> ADVGSCSVGNNPLAQLHKHTQQNKSLQFNQKNNGRLNESPLQGTNKPGISEAFISNVNAISQENMANMQRFINGEPLIDDKRRMEIGPSSGRLPPFSNVHSLQTSANPTQIKGVNDISHWSQEFQGSNSIQNRNADTGNSEKAWQRGSTTASSRFQYPNTMMNNYAYASMNSLSGSRLQSPAFMNQQQSGRSKEGVNEQEQQPWTDQFEKLEKEVSENLDINDEIEKEENVSEVEQNKPETVEKEEGVYGDQYQSDFQEVWDSIHKDAEEVLPSELVNDDLNLGEDYLKYLGGRVNGNIEYAFQSNNEYFNNPNAYKIGCLLMENGAKLSEAALAFEAAVKEKPDHVDAWLRLGLVQTQNEKELNGISALEECLKLDPKNLEAMKTLAISYINEGYDMSAFTMLDKWAETKYPEIWSRIKQQDDKFQKEKGFTHIDMNAHITKQFLQLANNLSTIDPEIQLCLGLLFYTKDDFDKTIDCFESALRVNPNDELMWNRLGASLANSNRSEEAIQAYHRALQLKPSFVRARYNLAVSSMNIGCFKEAAGYLLSVLSMHEVNTNN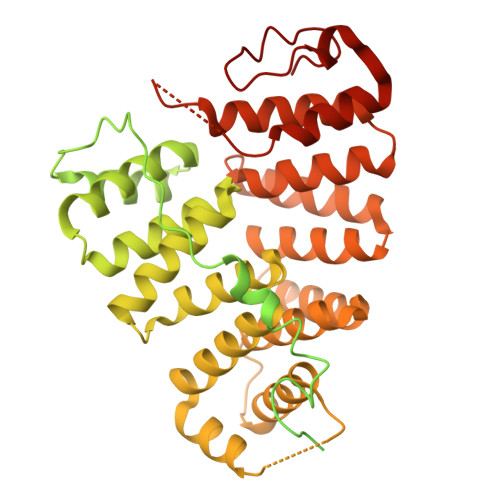KKGDVGSLLNTYNDTVIETLKRVFIAMNRDDLLQEVKPGMDLKRFKGEFSF>[4x]MLLAIDVRNTHTVVGLLSGMKEHAKVVQQWRIRTESEVTADELALTIDGLIGEDSER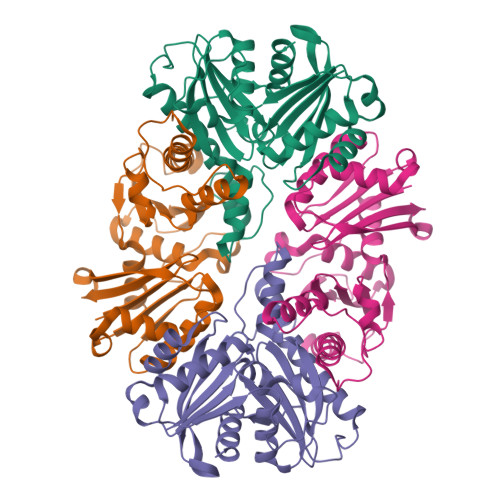LTGTAALSTVPSVLHEVRIMLDQYWPSVPHVLIEPGVRTGIPLLVDNPKEVGADRIVNCLAAYDRFRKAAIVVDFGSSICVDVVSAKGEFLGGAIAPGVQVSSDAAAARSAALRRVELARPRSVVGKNTVECMQAGAVFGFAGLVDGLVGRIREDVSGFSVDHDVAIVATGHTAPLLLPELHTVDHYDQHLTLQGLRLVFERNLEVQRGRLKTAR>[12x]MAALTPDLTTATPRLQYFHIAGPGTREYLSEDLQQFISATGSYFDLKNKFRQTVVAPTRNVTTEKAQRLQIRFYPIQTDDTSTGYRVRYNINVGDGWVLDMGSTYFDIKGILDRGPSFKPYCGTAYNPLAPKESMFNNWSETAPGQNVSASGQLSNVYTNTSTTKDTTAAQVTKISGVFPNPNQGPGINPLRQVENANTGVLGRFAKSQYNYAYGAYVKPVAADGSQSLTQTPYWIMNNAGTEYLGAVAVEDYTNSLSYPDTMIVPPPEDYDDYNIGTTRALRPNYIGFRDNFINLLYHDSGVCSGTLNSERSGMNVVVELPDRNTELSYQYMLADMMSRHHYFALWNQAVDQYDPEVRVFSNDGYEEGAPSYAFNPEAVGAGEGYG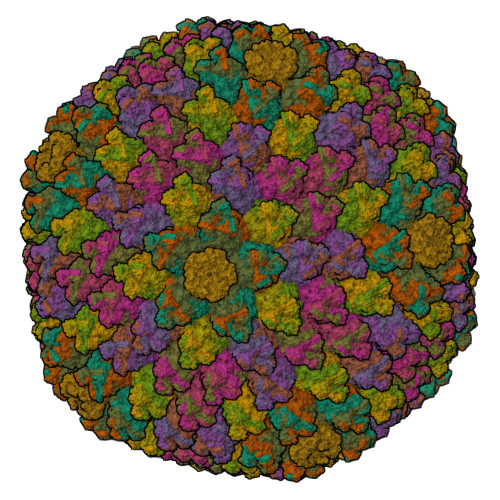PDLSQIKLYTNNTAANDKNTAVTNATTNFYFGTVPSYEIDISATQRRNFIMANIAEYLPDRYKFSISGFDATSVAPTTYEYMNKRVPLTNVVDMFTNVGARWSIDQMDNVNPFNHHRNWGLKYRSQLLGNSRYVNFHIQVPQKFFAIKNLLLLSGSYTYEWVLRKDPNMILQSSLGNDLRADGASIIYNEVNLMANFMPMDHNTSNQLELMLRNATNDQTFVDYLGAKNALYSVPAGSTALTINIPARTWEGMRGWSFTRIKAAETPQLGAQYDVNFKYSGSIAYSDGGFYLSHTFRNMSILFDTSINWPGNDRLLTPNMFEIKRSVALDTEGFTMSQCDITKDWYLIQMATNYNFVYNGYRFWPDRQYFHYDFLRNFDPMTRQGPNFALPGLFDLVSYTPTTDNSGEQPSQEAVRNNSGFIAPRSWPVWSAHQGESWPANWPYPLCGQQAIQPGQVLSYKKFLCDNYLWTIPFSSDFMYMGELTDLGQNPMYTNNSHSMVINFELDPMDDPTYVYMLYGVFDTVRVNQPERNVLAMAYFRTPFATGNAV;> MWGLQPPTSIPPPPPPTELTPSTYPAMVNGYPPPAASAQSCSSSGGQSELYMPLQRVMAPTGGRNSIKYRDYTPCRNTTKLFYVDNKASDIDTYNKDANHSNFRTTVIHNQDLDADTAATESIQLDNRSCWGGDLKTAVRTNCPNVSSFFQSNSVRVRMMWKRDPPTSTAPPSAVGSGYSVPGAQYKWYDLTVPEGNYALCELIDLLNEGIVQLYLSEGRQNNVQKSDIGVKFDTRNFGLLRDPVTGLVTPGTYVYKGYHPDIVLLPGCAIDFTYSRLSLLLGIGKREPYSKGFVITYEDLQGGDIPALLDLDSVDVNDADGEVIELDNAAPLLHDSAGVSYNVIYDQVTGKPVTAYRSWMLAYNVPNSQANQTTLLTVPDMAGGIGAMYTSLPDTFIAPTGFKEDNTTNLCPVVGMNLFPTYNKIYYQAASTYVQRLENSCQSATAAFNRFPENEILKQAPPMNVSSVCDNQPAVVQQGVLPVKSSLPGLQRVLITDDQRRPIPYVYKSIATVQPTVLSSATLQ;> MSSTEVFGALAPVGRTEVADALSSHANSKDARSLRYEPYANRLIKLQTAMVPPKVDGTSERVAEVVKGLAEQGAIYPDQMGAIHSDLLNRVYTWNSMGVQESIQALVNDVIHGQNKVLQDELARTREIANASMLTRFFDSLYKTVDRGQRNFEGFKKLLRLFVNNVPNAEVYSSGGSFSLQINMGGQSQNINLTNAFDNLKDIWGARWDAVNNPRIGALLTPNTRALLFFVSTFYDYGSMEPGSYLDNLMRLYKEAIRADTDAEGDAIMELGDAGANLNLKFNQYKDTLNYLLQNKPSVPQTGPLEMSPEQESLFKYLMRQLRRALKDGVNSDIAISTMAQYVDPRLYTSNKVFIDKLQNYLLMASARNPYYYKTIVLDPHWVPPAGLYTDNFVIPEMMPNFSDFASELEYGGPSRDEYFDDSPFRPPPQKKFTEKEQADYDSLINFFDSTLGVQSEAGWIADHRLPQAFDGALNVSERTPYNTPLPDDAPMRSRNASVSSATDALGQLKLSGTGGAGFFDSLKPSVGTRRSTGLAKGLAGTGQPPCPWPASVGYASAGYGPARGIRGSGLARRALAARGLRQGKRLRFY;>[2x]MNLLNAAPTPYVWKYNPVTGKCAGAQQNYGATIDWVLPGGNSFAYAADEIRRRFPEPAVTRAITARFEAESDQQPYAGPHETNIITADVVRSGPPPSAVYPFDPSGVQRVQLSGGMMGGRTEGRMQLSGGLTEGRMQLAGGAAGKLPTRARPTLRPPRWCGTTLTGNGLPADYPEMTPDAFKYYLRVQGPSQEVDEPGVMSQRQFMTTFLPAMVPHPFDSESPDAFPAYFSSVYKGTNAFEPVFWQG>[2x]MDQEKELPTSNKIDVENG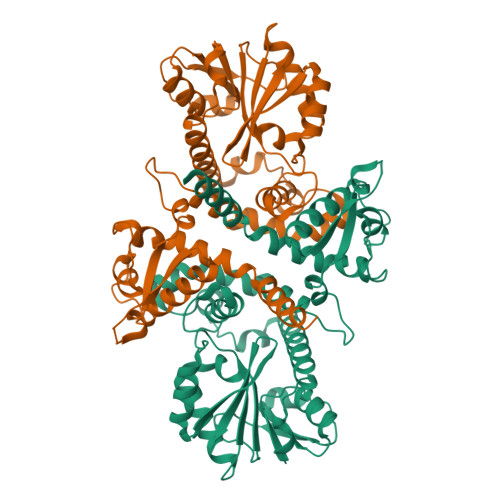DGSNRAEEEELCSYSNAIELAFSVVLPMVMKAAVELQVLDIIAKAGPRAQLSPSQIASQLPAAALRCSPDAPKMLDRMLCLLASHSILTCSAVDFHSDDHNDSPSTAAAALEDKRLYGLTPLAKYFVPNQDGVSLGPLMCLVQDKVCMKSWYELKGAVLEGGVPFMRVYGVESFDYPGTDPRFNEVLNNAMVNYSTIFLKKLMQSSYNGFEQVETLVDVGGGLGVALELITSKYPHIKAINFDLPHVIKHAKPYPGLEHVGGDMFESVPKGDAIFMKGVLHDWSDDLCLKLLKNCYKALPDNGKIIAVERILPEMPNSAGKGIFLMDLQMMTHHLGGRERTQQEYFDLAISAGFSGIRLECLVCNLWVIELYK>[2x]GSDSVITH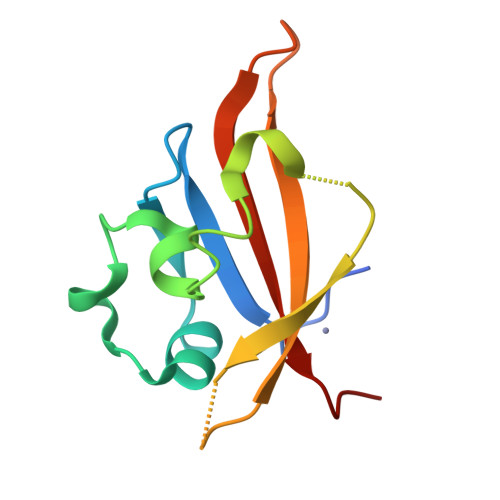MSDGIIATDRRGRIRIVNDMALKMLGMAKEDIIGYYMLSVLSLEDEFKLEEIQENNDSFLLDLNEEEGLIARVNFSTIVQETGFVTGYIAVLHDVTEQQ> MSPFLYLVLLVLGLHATIHCASPEGKVTACHSSQPNATLYKMSSINADFAFNLYRRFTVETPDKNIFFSPVSISAALVMLSFGACCSTQTEIVETLGFNLTDTPMVEIQHGFQHLICSLNFPKKELELQIGNALFIGKHLKPLAKFLNDVKTLYETEVFSTDFSNISAAKQEINSHVEMQTKGKVVGLIQDLKPNTIMVLVNYIHFKA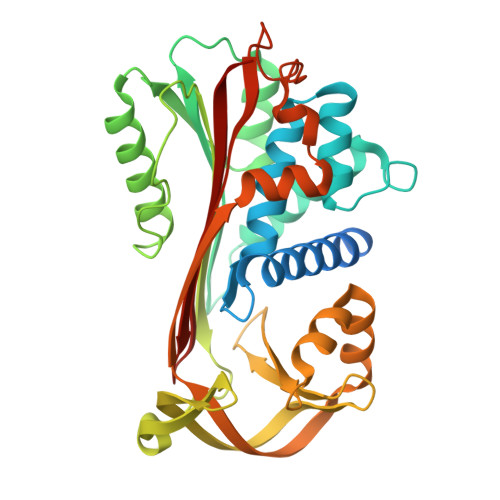QWANPFDPSKTEDSSSFLIDKTTTVQVPMMHQMEQYYHLVDMELNCTVLQMDYSKNALALFVLPKEGQMESVEAAMSSKTLKKWNRLLQKGWVDLFVPKFSISATYDLGATLLKMGIQHAYSENADFSGLTEDNGLKLSNAAHKAVLHIGEKGTEAAGAMFLEAIPR> NISVGRGRARLI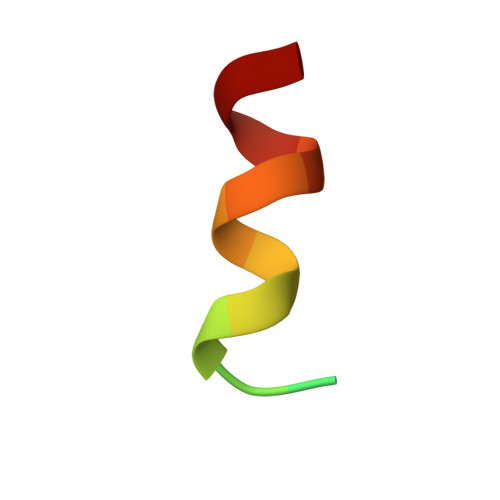DTLK> MGVRLYSCDACPHAVFTTHAALLAHAEEHHADLLPDHARLRRIAQKLNPVWNRALNARRNTITSWGKKIFHVAAQRDAGESKMQEAHRARAQLECVVRRWHDKARVFIFGSSVAMGVWDGTADIDFAVVDVDAMERGSWPPLEKNAVRSITELLRRVGFSFVNLEPISHARVPIIKHHASSPILTVARRDAEDVVARSIRFILNGPATREDRLLLEG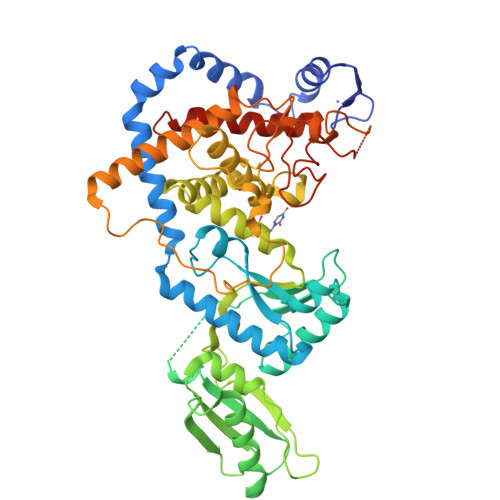SVRDAVGPTGVQQVWWNRTSDMMSATLESTTAAVRAAMCSPALASASLRTKVQPAHDECRPELYNIDFDLSFRAFGIRNSTLLRKYLLSHPCARPGAIVLKDWSKTSGVNNSVNGYFTSYAINIMWIYYLVQKGYVPYVDPLEIPESLVNYTDFDPRYTPMIDPEITNTEREELYKAAGDMLVGFFYFYSFEFDWGHNVISLNRPGITTKRMLGWHVEDVVPVASTSVSSGGGGSNVKRHPTRYELCIEDPYEENLNLGRHIGVTKSLRVRTELYRGLLSLLKEGETRSCVFAAA> DNL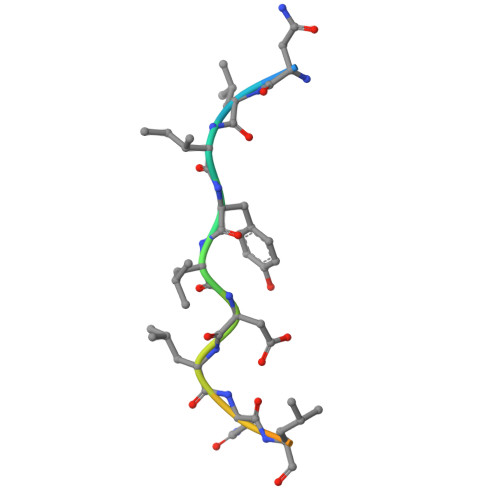IYLDLNLQDWDD>[4x]MRLHIALSLFYTLGHAVGAEPQHAKRTPKCRCTPGEACWPDNSVWEAFDKTLGKGKLIKTSPIAQSCYDGPQKDLDRCAYVNKMWTDQDFQTSDPIGRNYPYNITCAPVDYAAGETPTSCILGSLPYYAVNASTREDITLTLNFAKQHNIRLVTSSTGHDLLGRSDGYGGLELWLHSFRNGVRFQKKYTSANKCTKSGWTGSAIHIDGAYQWRDVYTVAQANNVIAVGGGSPSPGAIGGWPSGGGHGPATHNFGLGADQVLEAQIMLADGRIVTANHCENSDLFRAIRGGGPGYGIVLSQHIKVHPNVKAVTAHRLAIAPRNETAENKD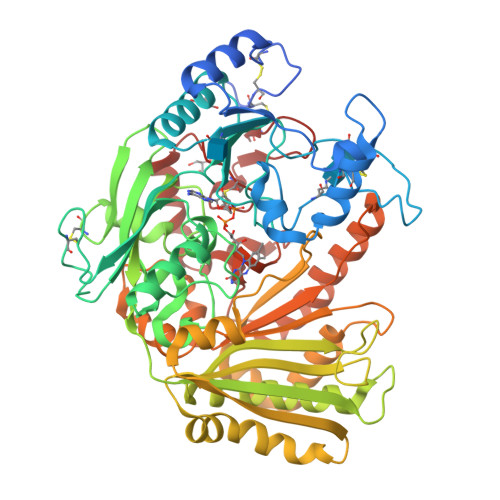LLDAIAVLHQQLPALSNNGVAGYGFWFRSFPGPFVGDAHSGYTHGFWTIGKRQAEAEKAVAPLMNALKKFEDKLVITSTFAEYQDYWSFYWAESGLHDPVGSTSIITSRLINPEALTDYNKVREAIEVVAGKPEEVSSNVVLLVSGGQVFKDKADTSSGLHPAWRVSPFVMISGQGIPKVASREIRDYVQHQVTHVKGAALKKLAPNTGGYMNEGDGSDPEYIDAFYGKNYAQHLAAKRKYDPDNIFFCRTCVGAEDFIERPDGPLCRK>CSLPGLSAAADQTIKIGAQSMSESEIIASMQGQLIEHHTDLKTTTIKNLGSNAVQQQALMNGEIDIAATRYTGDALTGTLRMEPEKDPDKALALTQREFKKRYDLKWYDSYGFDNTYAFTVSKELADQYHLETVSDVKKWAPQLKLGVDNYWMKLKGNGYQDFTKTYGMTFGGTYPMQIGLVYDAVKSGKMDIVLAYSTDGRIKSYGLKMLKD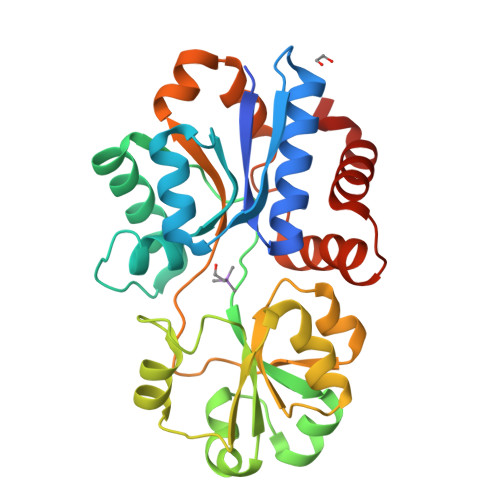DKQFFPPYDCSPVVPEKVLKEHPELEGIIKKMLGKIDTATMQELNYEVDGNLKEPSVVAKEYLEKHRYFES[2x]> MKKAVINGEQIRSISDLHQTLKKELALPEYYGENLDALWDALTGWVEYPLVLEWRQFEQSKQLTENGAESVLQVFREAKAE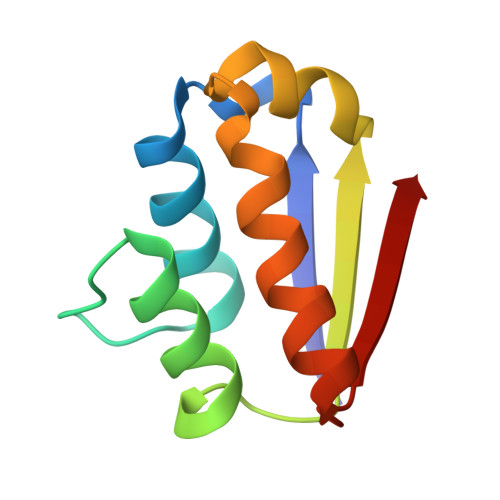GADITIILS Casitas B-lineage lymphoma (Cbl or c-Cbl) is a RING ubiquitin ligase that negatively regulates protein tyrosine kinase (PTK) signalling. The conserved N-terminus of Cbl family proteins contains a substrate tyrosine kinase-binding domain (TKBD), a linker helix region (LHR) and a RING domain. The RING domain mediates the transfer of ubiquitin (Ub) from an E2 Ub-conjugating enzyme to the substrate. Phosphorylation of a conserved residue (Tyr371) on the linker helix region (LHR) between the substrate-binding and RING domains is required to ubiquitinate PTKs, thereby flagging them for degradation.

Tyr371 is on the LH, and, in the unphosphorylated state, Tyr371 and several other residues from the LH, including Tyr368, bind to the TKBD, limiting movement between the RING and TKBD to rotation about LL2. In the native state, Trp258, Ala262, Val263, and Met274 form a hydrophobic pocket around the aromatic ring of Tyr371 and the side chain of Ser227 forms a hydrogen bond with the hydroxyl group of Tyr371. We predict that, while a large aromatic residue like Phe cannot duplicate the Tyr371-TKBD interactions, neither will it perturb those interactions; hence, Cbl Y371F can adopt and readily maintain conformations observed in the unphosphorylated state. In contrast, when Tyr371 is substituted with Phe, the UbcH5B–Ub binding affinity is comparable to wild-type (N-Cbl Y371F, 84 μM) and the LHR-TKBD interaction is unperturbed, as demonstrated by the crystallographic structure of N-Cbl Y371F. When Tyr371 is mutated to Phe, the hydrophobic interactions are not disturbed and the native state is maintained: the UbcH5B–Ub binding affinity, Rg, Dmax and Rflex values are comparable to native Cbl. Notably, N-Cbl Y371F appears slightly more compact and less flexible than wild-type N-Cbl, with an Rg of 2.38 nm, a Dmax of 7.67 nm, and an Rflex of approximately 56 %. In addition, previous in vitro autoubiquitination assays show native Cbl and Cbl Y371F have comparable catalytic efficiencies. Thus, in solution, it appears as though Cbl Y371F mimics the behaviour of native Cbl. Cbl Y368F is slightly more flexible than native Cbl but retains the ability to ubiquitinate receptor PTKs, whereas Cbl Y371F cannot ubiquitinate receptor PTKs but is able to maintain the native conformation in solution. For Cbl Y371F, neither the number of foci nor the relative cell density are significantly different than in cells infected with wild-type Cbl; these results suggest this mutant may potentiate transformation but not to the same extent as the other Cbl Y371 mutants or Cbl70Z.

>[6x]GSPPGTVDKKMVEKCWKLMDKVVRLCQNPKLALKNSPPYILDLLPDTYQHLRTILSRYEGKMETLGENEYFRVFMENLMKKTKQTISLFKEGKERMYEENSQPRRNLTKLSLIFSHMLAELKGIFPSGLFQGDTFRITKADAAEFWRKAFGEKTIVPWKSFRQALHEVHPISSGLEAMALKSTIDLTCNDYISVFEFDIFTRLFQPWSSLLRNWNSLAVTHPGYMAFLTYDEVKARLQKFIHKPGSYIFRLSCTRLGQWAIGYVTADGNILQTIPHNKPLFQALIDGFREGFYLFPDGRNQNPDLTGLCEPTPQDHIKVTQEQYELFCEMGSTFQLCKICAENDKDVKIEPCGHLMCTSCLTSWQESEGQGCPFCRCEIKGTEPIVVDPFD>SNAMKERVIITGANGQLGKQLQEELNPEEYDIYPFDKKLLDITNISQVQQVVQEIRPHIIIHCAAYTKVDQAEKERDLAYVINAIGARNVAVASQLVGAKLVYISTDYVFQGDRPEGYDEFHNPAPINIYGASKYAGEQFVKELHNKYFIVRTSWLYGKYGNNFVKTMIRLGKEREEISVVADQIGSPTYVADLNVMINKLIHTSLYGTYHVSNTGSCSWFEFAKKIFSYANMKVNVLPVSTEEFGAAAARP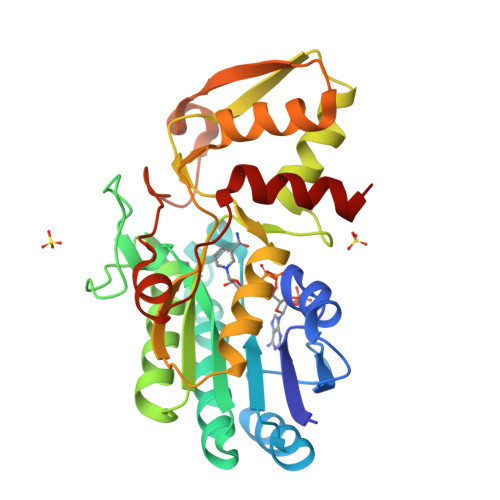KYSIFQHNMLRLNGFLQMPSWEEGLERFFIETKSH[6x]> VQDCYHGDGQSYRGTSSTTTTGKKCQSWSSMTPHRHQKTPENYPNAGLTMNYCRNPDADKGPWCFTTDPSVRWEYC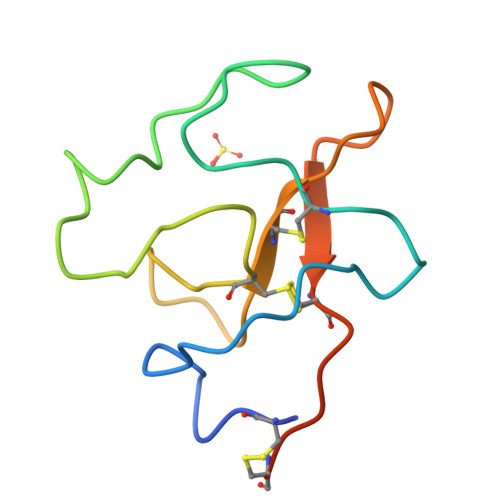NLKKCSGTEASV>[2x]MSLG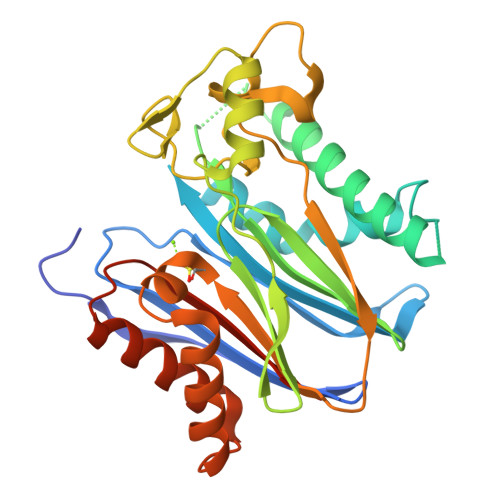AFLDKPKTEKHNAHGAGNGLRYGLSSMQGWRVEMEDAHTAVVGIPHGLEDWSFFAVYDGHAGSRVANYCSTHLLEHITTNEDFRAAGKSGSALELSVENVKNGIRTGFLKIDEYMRNFSDLRNGMDRSGSTAVGVMISPKHIYFINCGDSRAVLYRNGQVCFSTQDHKPCNPREKERIQNAGGSVMIQRVNGSLAVSRALGDYDYKCVDGKGPTEQLVSPEPEVYEILRAEEDEFIILACDGIWDVMSNEELCEYVKSRLEVSDDLENVCNWVVDTCLHKGSRDNMSIVLVCFSNEGHHHHHH The Arabidopsis VEL proteins are accessory proteins that interact with PRC2 to nucleate and propagate silencing at the FLOWERING LOCUS C (FLC) locus, enabling early flowering in spring. Here, we report that VEL proteins contain a domain related to an atypical four-helix bundle that engages in spontaneous concentration-dependent head-to-tail polymerization to assemble dynamic biomolecular condensates. The VEL domain adopts a compact globular fold, consisting of four α-helices in a quasi-antiparallel “up-down-up-down” configuration, each of which contributes to the hydrophobic core, as illustrated by VEL1VEL. Mutations blocking polymerization of this VEL domain prevent Polycomb silencing at FLC.

To test the function of VEL polymerization in FLC silencing in plants, we generated WT and mutant VIN3-GFP transgenes bearing R556D and I575D (RI>DD) for stable transformation of the Arabidopsis null mutant vin3-1 FRI. We confirmed by SEC-MALS that the polymerization of this double mutant is completely disabled. VIN3VEL crystals also show protofilaments; however, these are invariably composed of dimers rather than monomers as in VEL1VEL. Indeed, dimers are seen in every single crystal, regardless of the mutant, space groups, or crystallization conditions. Interestingly, these dimers result from mutual domain swapping of H4 between individual VIN3VEL monomers whereby molecule A donates its H4 to molecule B in an adjacent VIN3VEL filament, and vice versa. In contrast, the RI>DD transgene did not complement the FLC silencing defect of vin3-1 FRI, resulting in derepression of FLC, with high FLC transcript levels comparable to those seen in the null vin3-1 FRI mutant; importantly, the defective FLC silencing in the RI>DD rescue lines occurred both during and after cold exposure (orange).

>KDLGHIVKTIRCLEEEGHIDKSFREDFLTWYSLRATHREVRVVKDFVETFMEDLSSLGQQLVDTFSESILSKK[2x]Signaling through RET plays essential regulatory roles in the development of the nervous system and kidney. Glia cell line-derived growth factor (GDNF), Neurturin (NRTN), Artemin (ARTN) and Persephin are four ligands that induce dimerization of RET through assembling 2:2:2 ternary complexes with RET and the co-receptors GDNF receptor-α family proteins (GFRα1–4). Here, we report the cryo-EM structures of four extracellular 2:2:2 ligand/co-receptor/RET complexes, including GDF15/GFRAL/RET, GDNF/GFRα1/RET, NRTN/GFRα2/RET and ARTN/GFRα3/RET, at near-atomic resolution. The structures show that the extracellular region of RET adopts a ‘C-clamp’ shape, which is stabilized by extensive inter-domain interactions as well as binding of calcium ion at multiple sites.

The same procedure was used for the structure determination of the 2:2:2 NRTN/GFRα2/RET and ARTN/GFRα3/RET complexes, leading to reconstructions to 3.4 Å and 3.5 Å resolution, respectively. A recently published medium resolution (5.7 Å) cryo-EM structure of the NRNT/GFRα2/RET complex displays a similar overall architecture. The segments in GFRα1, GFRα2 and GFRα3 corresponding to the helix-loop-helix-loop motif in GFRAL are much shorter and adopt extended loop conformations. As a result, interfaces I in GFRα1/RET, GFRα2/RET and GFRα3/RET are much smaller (buried surface areas less than 700 Å2) and likely weaker than that in GFRAL/RET (buried surface area ~ 1500 Å2). In contrast, the D1 domain of GFRα2 is resolved in the cryo-EM map of the NRTN/GFRα2/RET complex, and packs closely with the D3 domain as seen in the crystal structure of the NRTN/GFRα2 complex. The D1 domain of GFRα2 makes a few contacts with RET-CLD1, which may help stabilize the ternary complex. However, there are large differences in the angle between the two wings of the batwing-shaped complexes, which mainly originate from the different conformations of the ligand dimers and their different interfaces with the co-receptors. This angle in the GDF15/GFRAL/RET complex (~60°) is much more acute than that in the complexes of GDNF/GFRα1/RET (130°), NRTN/GFRα2/RET (105°) and ARTN/GFRα3/RET (108°).

>[2x]ARLGARPCGLRELEVRVSELGLGYASDETVLFRYCAGACEAAARVYDLGLRRLRQRRRLRRERVRAQPCCRPTAYEDEVSFLDAHSRYHTVHELSARECACV;>SSLQGPELHGWRPPVDCVRANELCAAESNCSSRYRTLRQCLAGRDRNTMLANKECQAALEVLQESPLYDCRCKRGMKKELQCLQIYWSIHLGLTEGEEFYEASPYEPVTSRLSDIFRLASIFSGTGADPVVSAKSNHCLDAAKACNLNDNCKKLRSSYISICNREISPTERCNRRKCHKALRQFFDRVPSEYTYRMLFCSCQDQACAERRRQTILPSCSYEDKEKPNCLDLRGVCRTDHLCRSRLADFHANCRASYQTVTSCPADNYQACLGSYAGMIGFDMTPNYVDSSPTGIVVSPWCSCRGSGNMEEECEKFLRDFTENPCLRNAIQAFGNGTDVNGTHHHHHHHH[2x];>[2x]LYFSRDAYWEKLYVDQAAGTPLLYVHALRDAPEEVPSFRLGQHLYGTYRTRLHENNWICIQEDTGLLYLNRSLDHSSWEKLSVRNHGFPLLTVYLKVFLSPTSLREGECQWPGCARVYFSFFNTSFPACSSLKPRELCFPETRPSFRIRENRPPGTFHQFRLLPVQFLCPNISVAYRLLEGEGLPFRCAPDSLEVSTRWALDREQREKYELVAVCTVHAGAREEVVMVPFPVTVYDEDDSAPTFPAGVDTASAVVEFKRKEDTVVATLRVFDADVVPASGELVRRYTSTLLPGDTWAQQTFRVEHWPNETSVQANGSFVRATVHDYRLVLNRNLSISENRTMQLAVLVNDSDFQGPGAGVLLLHFNVSVLPVSLHLPSTYSLSVSRRARRFAQIGKVCVENCQAFSGINVQYKLHSSGANCSTLGVVTSAEDTSGILFVNDTKALRRPKCAELHYMVVATDQQTSRQAQAQLLVTVEGSYVAEEAGCPLSCAVSKRRLECEECGGLGSPTGRCEWRQGDGKGITRNFSTCSPSTKTCPDGHCDVVETQDINICPQDCLRGSIVGGHEPGEPRGIKAGYGTCNCFPEEEKCFCEPEDIQDPLCDELCRGTHHHHHHHH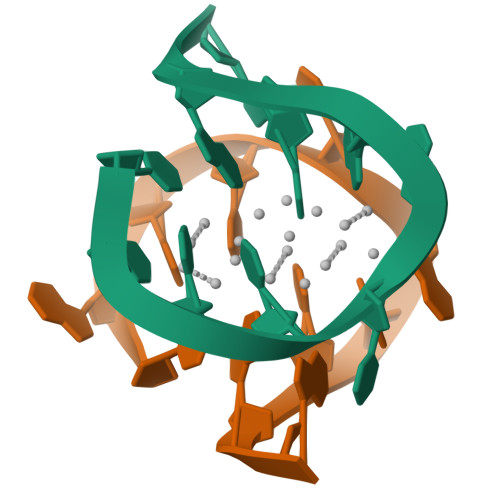>CACCTAICIA[12x]> MHHHHHHHMEQIAQQQPQTLCIKHLAKNYSKRWVVKDVSFEMQSGQIVGLLGPNGAGKTTSFYMVVGLVRMDKGEIHLDNLDLSDLAMHERARKGIGYLPQEASIFRKL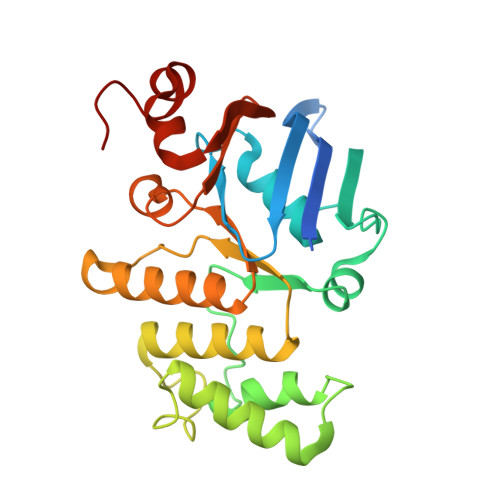TIAENIMAILETRKDLNKQQRQQRLQELLNDFKITHIKDSLGMSVSGGERRRAEIARALAADPKFMLLDEPFAGVDPISVGDIKDIIRNLKDRGIGVLITDHNVRETLAICEHAYIVSEGAVIAEGSPQDILENEQVRKVYLGDDFTV>[2x]ILTKHGKNPVMELNEKRRGLKYELISETGGSHDKRFVMEVEVDGQKFQGAGS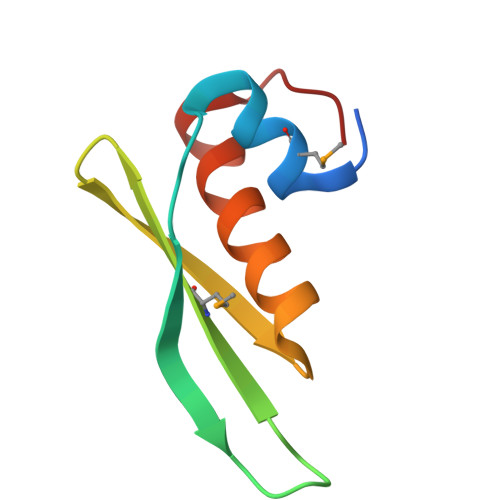NKKVAKAYAALAALEKLFPDTPL~{N}-ethyl-4-oxidanylidene-4-phenyl-butanamide | 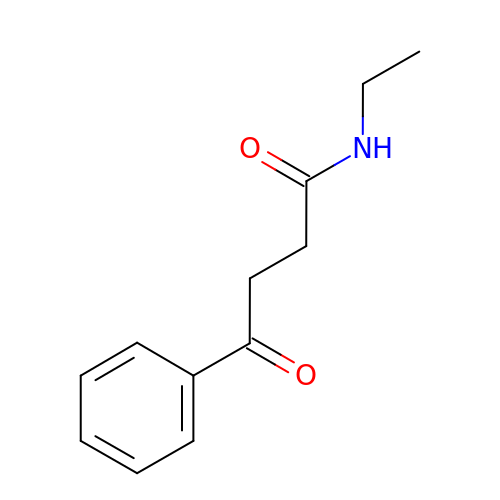C12 H15 N O2 | DSZHWKIWJYHWTO-UHFFFAOYSA-N> MVEATAQETDRPRFSFSIAAREGKARTGTIEMKRGVIRTPAFMPVGTAATVKALKPETVRATGADIILGNTYHLMLRPGAERIAKLGGLHSFMGWDRPILTDSGGFQVMSLSSLTKQSEEGVTFKSHLDGSRHMLSP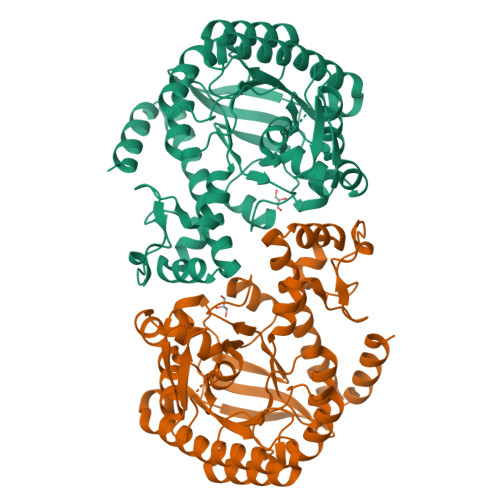ERSIEIQHLLGSDIVMAFDECTPYPATPSRAASSMERSMRWAKRSRDAFDSRKEQAENAALFGIQQGSVFENLRQQSADALAEIGFDGYAVGGLAGGEGQDEMFRVLDFSVPMLPDDKPHYLMGVGKPDDIVGAVERGIDMFDCVLPTRSGRNGQAFTWDGPINIRNARFSEDLKPLDSECHCAVCQKWSRAYIHHLIRAGEILGAMLMTEHNIAFYQQLMQKIRDSISEGRFSQFAQDFRARYFARNS>LQHQNPQQLSSNLWAAVRARGCQFLGPAMQEEALKLVLLALEDGSALSRKVLVLFVVQRLEPRFPQASKTSIGHVVQLLYRASCFKVTKRDEDSSLMQLKEEFRTYEALRREHDSQIVQIAMEAGLRIAPDQWS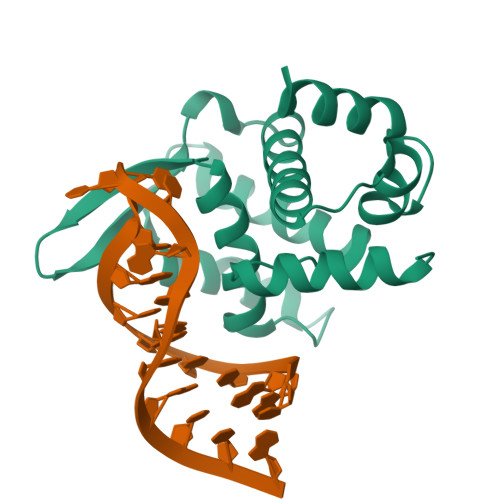SLLYGDQSHKSHMQSIIDKLQTPASFAQSVQELTIALQRTGDPANLNRLRPHLELL[4x]A key step in bacteriochlorophyll biosynthesis is the reduction of protochlorophyllide to chlorophyllide, catalyzed by dark-operative protochlorophyllide oxidoreductase. Like nitrogenase, DPOR is composed of two proteins: a homodimeric L-protein (BchL) and a heterotetrameric NB-protein (BchNB). BchL serves as the ATP-dependent electron donor, and BchNB is the electron acceptor containing the active site for Pchlide binding and reduction. Given the structural similarity to nitrogenase, ATP binding to BchL is thought to promote its transient association with BchNB followed by a single ET to Pchlide.

R. sphaeroides BchL was crystallized anaerobically in the absence of nucleotides, and a crystal structure was determined to a resolution of 2.6 Å. The asymmetric unit contains four BchL chains: chains A and B form one BchL dimer and chains C and D comprise the other. The overall conformations of the AB and CD dimers are highly similar (Cα RMSD, of 0.55 Å). Interestingly, in chain C, we observe the flexible N-terminus bound across the [4Fe-4S] cluster (dark blue) covering a surface that is normally used to interface with BchNB (purple). Although the electron density for this region is not observed in the other chains, superimposing chain C onto chain D reveals that only one N-terminus would be able to bind in the observed conformation because of steric clashes. For example, in chain C, Asp-23 forms a hydrogen bond with Gln-168 (bond distance of 2.8 Å), whereas the backbone oxygen of Gly-16 (chain C) is within hydrogen-bonding distance of the Cys-126 (chain D) backbone amide (3.5 Å), a [4Fe-4S] cluster-ligating residue. In addition, the side chain of Ser-17 (chain C) is well positioned to interact with the residue directly adjacent to Cys-126, Gly-125 of chain D, through a hydrogen bond with the backbone amide (3.5 Å). The position and specific interactions of the N-terminal residues in our nucleotide-free structure suggest a possible autoinhibitory role by forming a barrier to docking and shielding the [4Fe-4S] cluster of BchL. In the both the ADP-bound structure and our nucleotide-free structure, Asp-182 appears to form a weak hydrogen bond with Lys-39 of the same chain but does not interact with the other subunit.

>MGSSHHHHHHSQDPENLYFQSMSPKDLTIPTGADGEGSVQVHLDEADKITGAKVFAVYGKGGIGKSTTSSNLSAAFSILGKRVLQIGCDPKHDSTFTLTGSLVPTVIDVLKDVDFHPEELRPEDFVFEGFNGVMCVEAGGPPAGTGCGGYVVGQTVKLLKQHHLLDDTDVVIFDVLGDVVCGGFAAPLQHADQAVVVTANDFDSIYAMNRIIAAVQAKSKNYKVRLAGCVANRSRATDEVDRFCKETNFRRLAHMPDLDAIRRSRLKKKTLFEMDEDQDVLAARAEYIRLAESLWRGLDPIDPHSLPDREIFELLGFD[4x]> MDNGTDSSTSKFVPEYRRTNFKNKGRFSADELRRRRDTQQVELRKAKRDEALAKRRNFIPPTDGADSDEEDESSVSADQQFYSQLQQELPQMTQQLNSDDMQEQLSATVKFRQILSREHRPPIDVVIQAGVVPRLVEFMRENQPEMLQLEAAWALTNIASGTSAQTKVVVDADAVPLFIQLLYTGSVEVKEQAIWALGNVAGDSTDYRDYVLQCNAMEPILGLFNSNKPSLIRTATWTLSNLCRGKKPQPDWSVVSQALPTLAKLIYSMDTETLVDACWAISYLSDGPQEAIQAVIDVRIPKRLVELLSHESTLVQTPALRAVGNIVTGNDLQTQVVINAGVLPALRLLLSSPKENIKKEACWTISNITAGNTEQIQAVIDANLIPPLVKLLEVAE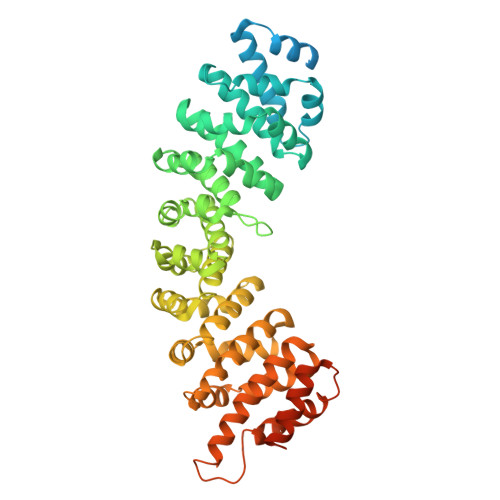YKTKKEACWAISNASSGGLQRPDIIRYLVSQGCIKPLCDLLEIADNRIIEVTLDALENILKMGEADKEARGLNINENADFIEKAGGMEKIFNCQQNENDKIYEKAYKIIETYFGEEEDAVDETMAPQNAGNTFGFGSNVNQQFNFN The DNA replication process is a desirable target for an antifungal product; hence, A. fumigatus proliferating cell nuclear antigen (afumPCNA) has been hypothesised as a fungal target for the development of new antifungals. The PCNA processivity factor is also known as the sliding clamp, as DNA slides through its central cavity. PCNA functions as a docking platform to allow DNA polymerases and a host of DNA replication and repair machinery to interact at the replication fork. The PCNA homotrimer comprises two domains, with each containing two alpha helices and nine beta strands, connected by a motif known as the interdomain connecting loop (IDCL), which forms part of the PCNA surface with which binding domain proteins interact.

The p21-derived peptide (139–160) was previously shown to bind to afumPCNA via fluorescence polarization with a KD of 3.1 µM. Previously, a shorter scaffold of this 22 amino acid p21 peptide was derived and synthesized: p21µ (141–155). It is 14 amino acids long, and it retained high-affinity binding, which was used to construct a library with variations relative to PIP-box residues as a rational starting point for the investigation of the fungal binding site. The co-crystal structure of afumPCNA bound to the p21µ peptide supports the hypothesis that A. fumigatus adopts a PIP-box sequence as a method for proteins to interact with afumPCNA. Here, we present an investigation of extensive structure–activity relationships between designed p21-based peptides and afumPCNA and the first crystal structure of a p21 peptide bound to afumPCNA, demonstrating that the A. fumigatus replication model uses a PIP-box sequence as the method for binding to afumPCNA. Differences in the protein sequence of afumPCNA and hPCNA account for the shift in affinity with the conservation of the secondary structure of the peptide. There is structural conservation around the 310 helical secondary structure and PIP-box, with more variability on the N- and C-terminus likely due to the mobility of the ends of the peptide and changes in IDCL residues. One prominent example is residue His125, which forms an antiparallel β-sheet with the C-terminal residues of p21 peptide on hPCNA (139–160); however, in the afumPCNA structure, afumPCNA His125 obstructs the formation of a favorable side chain hydrogen bond with the His152 side chain of the p21 peptide (139–160). This has the effect of pushing the C-terminus to be quite distant from the protein’s surface while not forming the hydrogen bonds of the β-sheet as observed in the human structure. There is also the loss of 3.4 Å hydrogen bond interactions between hPCNA Gln131 and the Tyr151 phenol of p21µ in afumPCNA as this residue is Thr131.

>MLEARLEQASLLKRVVDAIKDLVQDCNFDCNDSGIALQAMDNSHVALVSMLLKAEGFSAYRCDRNIALGINLVSLTKVLRAAQNEDILTLKADDSPDAVNLMFESAETDRISEYDIKLMDIDQEHLAIPETEYAATVEMPSAEFQRICRDLNALSESVVIEATKEGVKFSCQGDIGSGSVTIRQHTSVDKPEQNVSIALSEPVALTFSLKYLVNFCKATSLSSKVTLCLSQEVPLLVEYGLGSGHLRFYLAPKIGD[3x];>KRRQTSMTDFYHSKR[3x]> GAMDPMAYINIAEWTPDQVTDWIKGLDESMKGYLYEFSKQEIGGRALLNIRPYELENLGMLRIGHQEIVLEAVENLRNFHYHLKNDNLQFMALHVATAAKNLHRELA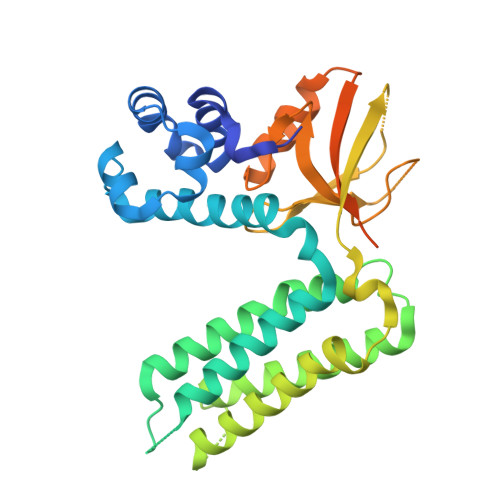RNHAESTKIDTRILHDITRTIATLKPLVGSLERTPFRKQEMYREYCGNVLKCGLELATIAHRDRFALQPVPAIRQSAERLENLANFVIQDISDPMVLQPASLNLVTLKKRESELGFNIESSYNGIHRVTDIKYNSPAHNSGKIEDGDEIVQINYQTVVGWQHRTVLEHLREALPDVVLTVKKRPKHTKMFGQIYMQPYRLPSKKRNMAARWAAQMPSPRAAFLTLDTE Human NAD-dependent isocitrate dehydrogenase or IDH3 (HsIDH3) catalyzes the decarboxylation of isocitrate into α-ketoglutarate in the tricarboxylic acid cycle. It consists of three types of subunits (α, β, and γ) and exists and functions as the (αβαγ)2 heterooctamer. HsIDH3 is regulated allosterically and/or competitively by numerous metabolites including CIT, ADP, ATP, and NADH. In this work, we report the crystal structures of the αβ and αγ heterodimers and the (αβαγ)2 heterooctamer containing an α-Q139A mutation in the clasp domain, which renders all the heterodimers and the heterooctamer constitutively active in the absence of activators.

Thus, we tried to crystallize the (αMβαMγ)2 holoenzyme in the absence of activators and finally were able to solve the crystal structure of the mutant holoenzyme with an active conformation at 4.5 Å resolution. The structure of the (αMβαMγ)2 holoenzyme belongs to space group C2221 and each asymmetric unit contains two (αMβαMγ)2 heterooctamers. The overall structure of the (αMβαMγ)2 holoenzyme is similar to that of the WT (αβαγ)2 holoenzyme. Intriguingly, when one heterotetramer of the two structures is superposed, the other heterotetramer of the mutant holoenzyme shows approximately 20° rotation relative to that of the WT holoenzyme. Moreover, in the mutant (αMβαMγ)2 structure, the active site and the allosteric site of the αγ heterodimer, the active site and the pseudo-allosteric site of the αβ heterodimer, and the αβ-αγ interface appear to assume active conformations. In particular, the N-terminal regions of the α7 helices in all of the α, β, and γ subunits assume helical conformations similar to that in the active αMgγMg+CIT structure. In addition, the sidechains of Tyr126A and Tyr137B in the αMβ heterodimer adopt active conformations; and while the sidechain of Tyr136G in the αMγ heterodimer is not clearly defined in the electron density map, the sidechain of Tyr126A also adopts active conformation. In other words, the α-Q139A mutation induces conformational changes of the clasp domains of the α subunits and the αβ-αγ interface and subsequently the active sites, the allosteric sites, and the pseudo-allosteric sites, which mimic the conformational changes induced by the binding of activators at the allosteric site, rendering the mutant holoenzyme to adopt the active conformation. Nevertheless, as the resolution of the (αMβαMγ)2 structure is low, we could not perform detailed structural analysis of the αβ-αγ interface and compare it with that in the inactive WT (αβαγ)2 structure. Moreover, the size-exclusion chromatography–multiangle light scattering (SEC-MALS) analysis shows that similar to the WT holoenzyme, the mutant holoenzyme displays an average mass of approximately 290 kDa at both low concentration (1 mg/ml) and high concentration (10 mg/ml) corresponding to an (αMβαMγ)2 heterooctamer.

>[8x]TGGVQTVTLIPGDGIGPEISAAVMKIFDAAKAPIQWEERNVTAIQGPGGKWMIPSEAKESMDKNKMGLKGPLKTPIAAGHPSMNLLLRKTFDLYANVRPCVSIEGYKTPYTDVNIVTIRENTEGEYSGIEHVIVDGVVASIKLITEGASKRIAEFAFEYARNNHRSNVTAVHKANIMRMSDGLFLQKCREVAESCKDIKFNEMYLDTVCLNMVQDPSQFDVLVMPNLYGDILSDLCAGLIGGLGVTPSGNIGANGVAIFESVHGTAPDIAGKDMANPTALLLSAVMMLRHMGLFDHAARIEAACFATIKDGKSLTKDLGGNAKCSDFTEEICRRVKDLD;>ASRSQAEDVRVEGSFPVTMLPGDGVGPELMHAVKEVFKAAAVPVEFQEHHLSEVQNMASEEKLEQVLSSMKENKVAIIGKIHTPMEYKGELASYDMRLRRKLDLFANVVHVKSLPGYMTRHNNLDLVIIREQTEGEYSSLEHESARGVIECLKIVTRAKSQRIAKFAFDYATKKGRGKVTAVHKANIMKLGDGLFLQCCEEVAELYPKIKFETMIIDNCCMQLVQNPYQFDVLVMPNLYGNIIDNLAAGLVGGAGVVPGESYSAEYAVFETGARHPFAQAVGRNIANPTAMLLSASNMLRHLNLEYHSSMIADAVKKVIKVGKVRTSDMGGYATCHDFTEEICRRVKDLDEN[4x];>[4x]FSEQTIPPSAKYGGRHTVTMIPGDGIGPELMLHVKSVFRHACVPVDFEEVHVSSNADEEDIRNAIMAIRRNRVALKGNIETNHNLPPSHKSRNNILRTSLDLYANVIHCKSLPGVVTRHKDIDILIVRENTEGEYSSLEHESVAGVVESLKIITKAKSLRIAEYAFKLAQESGRKKVTAVHKANIMKLGDGLFLQCCREVAARYPQITFENMIVDNTTMQLVSRPQQFDVMVMPNLYGNIVNNVCAGLVGGPGLVAGANYGHVYAVFETATRNTGKSIANKNIANPTATLLASCMMLDHLKLHSYATSIRKAVLASMDNENMHTPDIGGQGTTSEAIQDVIRHIRVINGRAVEA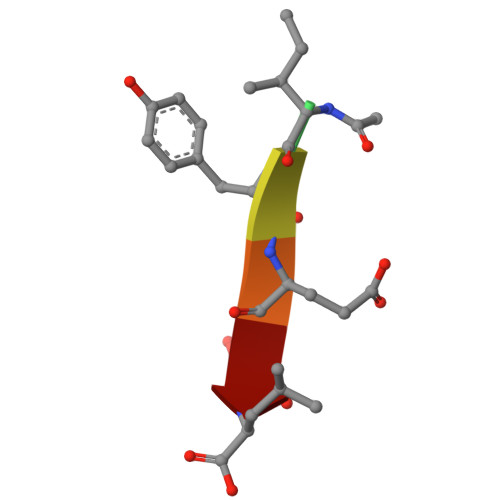> XIYESL> QGTLLVLHGP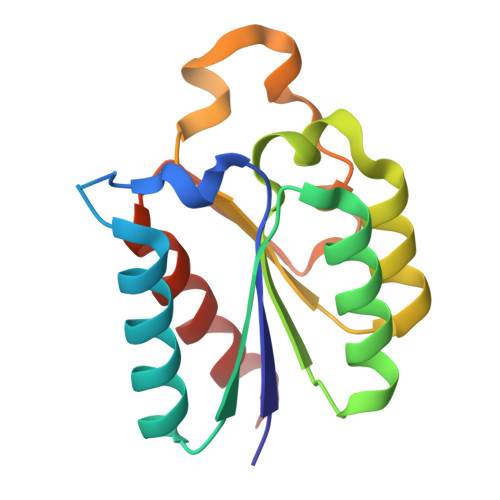NLNLLGTREPGTYGSTTLGQINQDLERRAREAGHHLLHLQSNAEYELIDRIHAARDEGVDFIIINPAAFTHTSVALRDALLAVSIPFIEVHLSNVHKREPFRHHSYFSDVAVGVICGLGATGYRLALESALEQLQ> MSTINNQLKALKVIPVIAIDNAEDIIPLGKVLAENGLPAAEITFRSSAAVKAIMLLRSAQPEMLIGAGTILNGVQALAAKEAGATFVVSPGFNPNTVRACQIIGIDIVPGVNNPSTVEAALEMGLTTLKFFPAEASGGISMVKSLVGPYGDIRLMPTGGITPSNIDNYLAIPQVLACGGTWMVDKKLVTNGEWDEIARLTREIVEQVNPG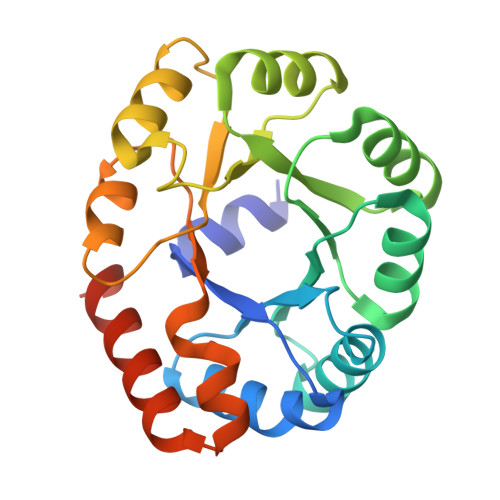SLEHHHHHH> GAMGEDVDKTLNELLAAEDTDKNYQITIEDTGPKVLKVGTANSYGYKHINIRGTYMLSNLLQELTIAKSFGRHQIFLDEARINENPVNRLSRLINTQFWNSLTRRVDLNNVGEIAKDTKIDTPGAKNPRIYVPYDCPEQYEFYVQASQMHPSLKLEVEYLPKKITAEYVKSVNDTPGLLALAMEEHFNPSTGEKTLIGYPYAVPGGRFN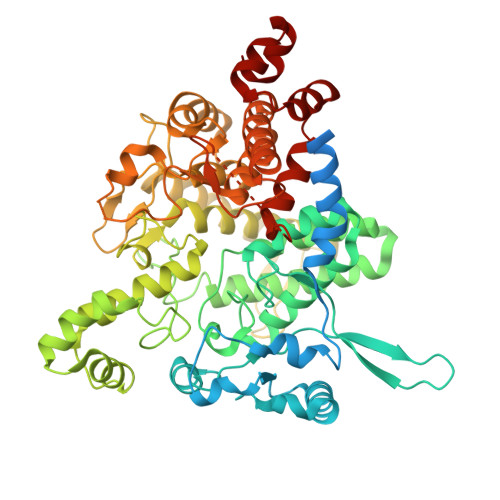ELYGWDSYMMALGLLEANKTDVARGMVEHFIFEINHYGKILNANRSYYLCRSQPPFLTEMALVVFKKLGGRSNPDAVDLLKRAFQASIKEYKTVWTASPRLDPETGLSRYHPNGLGIPPETESDHFDTVLLPYASKHGVTLDEFKQLYNDGKIKEPKLDEFFLHDRGVRESGHDTTYRFEGVCAYLATIDLNSLLYKYEIDIADFIKEFCDDKYEDPLDHSITTSAMWKEMAKIRQEKITKYMWDDESGFFFDYNTKIKHRTSYESATTFWALWAGLATKEQAQKMVEKALPKLEMLGGLAACTERSRGPISISRPIRQWDYPFGWAPHQILAWEGLRSYGYLTVTNRLAYRWLFMMTKAFVDYNGIVVEKYDVTRGTDPHRVEAEYGNQGADFKGAATEGFGWVNASYILGLKYMNSHARRALGACIPPISFFSSLRPQERNLYGL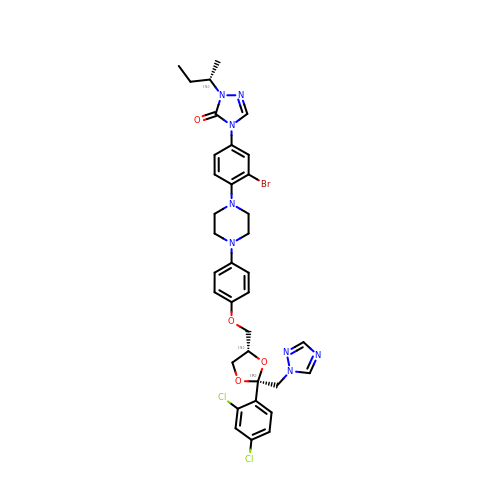4-(3-bromo-4-{4-[4-({(2R,4S)-2-(2,4-dichlorophenyl)-2-[(1H-1,2,4-triazol-1-yl)methyl]-1,3-dioxolan-4-yl}methoxy)phenyl]piperazin-1-yl}phenyl)-2-[(2S)-butan-2-yl]-2,4-dihydro-3H-1,2,4-triazol-3-one | C35 H37 Br Cl2 N8 O4 | NLXNHAVZBIVNIU-DIDXUJGESA-N> MPFTIDSARGIFPNTLAADVVPATIARFSQLNAEDQLALIWFAYLEMGKTLTIAAPGAASMQLAENALKEIQAMGPLQQTQAMCDLANRADTPLCRTYASWSPNIKLGFWYRLGELMEQGFVAPIPAGYQLSANANAVLATIQGLESGQQITVLRNAVVDMGFTAGKDGKRIAEPVVPPQDTASRTKVSIEGVTNATVLNYMDNLNANDFDTLIELFTSDGALQPPFQRPIVGKENVLRFFREECQNLKLIPERGVTEPAEDGFTQIKVTGKVQTPWFGGNVGMNIAWRFLLNPEGKIFFVAIDLLASPKELLNFAR

A kind of “molecular surgery” with “atomic mutations” is required to remove or replace individual atoms or groups of atoms in the context of complex proteins containing thousands of atoms with a complicated network of, for example, covalent, non-covalent or hydrogen bonding and van der Waals interactions. It has been suggested that the function of the Orange Carotenoid Protein (OCP), a blue light-driven photoswitch involved in photoprotection of cyanobacteria, strongly depends on two critical H-bonds between the ketocarotenoid cofactor and a tryptophan (Trp) and a tyrosine (Tyr) residue in the surrounding protein matrix. Structurally, the 35 kDa OCP consists of an N-terminal domain (NTD) composed entirely of α-helices and a mixed α/β-type C-terminal domain (CTD) of about equal size, both encapsulating a single ketocarotenoid molecule in a common central cavity. Upon absorption of a photon, OCP converts from the dark-adapted, orange OCPO state to the red, active OCPR state. By exposing the chromophore to the terminally emitting pigments of the PBSs, OCPR acts as an efficient quencher of PBS fluorescence, protecting the underlying photosystems from the deleterious effects of overexcitation and dissipating the electronic excitation energy into heat.

To this end, we used a recently evolved orthogonal pair consisting of a custom-tailored Methanosarcina mazei pyrrolysine tRNA synthetase (MmPylRS) and its cognate tRNA to replace Trp288 in OCP with 3-benzothienyl-L-alanine (BTA), an isostructural analogue of tryptophan in which the imino nitrogen is substituted by a sulphur atom. The resulting OCP-W288_BTA protein is photoactive and, according to the X-ray crystal structure solved at 1.8 Å resolution, fully isomorphous to the wild-type protein, allowing us to parametrize the consequences of the absence of a single H-bond by spectroscopic, thermodynamic and computational methods. As expected, the overall structure is very similar to the wild-type OCP, with RMSD values of 0.180 Å and 0.203 Å for monomer and dimer alignments at the Cα-positions, respectively. A close inspection of Figure 5A clearly shows that the BTA mutation has no significant effect on the global OCP structure, and the different geometry of the BTA side chain (C-S-C angle of 92.5°) compared to Trp288 (C-N-C angle of 109°) is nicely reflected by the electron density. The introduced BTA residue matches well with its native Trp288 counterpart, resulting in an almost identical spatial arrangement (i.e., isomorphic replacement). Interestingly, the distance to the keto oxygen atoms of the ECN/CAN cofactors increases only slightly from 2.9 Å in the wild-type protein to 3.2 Å and 3.3 Å, respectively, despite the potential repulsion of the lone electron pairs of sulphur, which, however, do not appear as a significant electron density in the 2mFo-DFc map. In addition, the distance between Tyr201 and the keto oxygen of ECN and is almost identical at 2.5 Å compared to 2.6 Å in wild-type OCP.>MGASKLRAVLEKLKLSRDDISTAAGMVKGVVDHLLLRLKCDSAFRGVGLLNTGSYYEHVKISAPNEFDVMFKLEVPRIQLEEYSNTRAYYFVKFKRNPKENPLSQFLEGEILSASKMLSKFRKIIKEEINDIKDTDVIMKRKRGGSPAVTLLISEKISVDITLALESKSSWPASTQEGLRIQNWLSAKVRKQLRLKPFYLVPKHAKEGNGFQEETWRLSFSHIEKEILNNHGKSKTCCENKEEKCCRKDCLKLMKYLLEQLKERFKDKKHLDKFSSYHVKTAFFHVCTQNPQDSQWDRKDLGLCFDNCVTYFLQCLRTEKLENYFIPEFNLFSSNLIDKRSKEFLTKQIEYERNNEFPVFDEF[2x]

Cyclic GMP‐AMP synthase (cGAS)* is a sensor of cytosolic double‐stranded DNA (ds‐DNA). ds‐DNA in the cytosol may occur from infection or mitochondrial damage. cGAS is activated by ds‐DNA binding to catalyze the cyclization of ATP and GTP to form a cyclic dinucleotide with mixed 2′,5′‐ and 3′,5′‐phosphodiester linkage (2′,3′‐cGAMP), which in turn activates stimulator of type 1 interferon genes (STING). Activated STING causes the activation of TBK1, which phosphorylates IRF3 allowing it to translocate to the nucleus where it triggers interferon‐inducible gene activation and interferon production. We report here the structure of cGAS with dinucleotides and small molecule inhibitors, and kinetic studies of the cGAS mechanism.

To study the β‐pseudo‐active form we obtained structures of an N‐terminal truncation of cGAS starting at residue 161 (cGAS161)22 in complex with five cyclic dinucleotides (2′,2′‐cGAMP, 2′,3′‐cGAMP, 3′,3′‐cGAMP, 3′,3′‐cdIMP and 3′,3′‐cdUMP), and the linear 2′,5′‐GpAp dinucleotide. In four of these structures, cGAS assumes the β‐pseudo‐active conformation. There is always an interaction between the catalytic acid Asp227 and the dinucleotide when the β‐pseudo‐active conformation occurs. In most cases Asp227 forms a hydrogen bond with the amino group of the guanine base with an approach between 2.5 and 3.3 Å. The exception to this is 3′,3′‐cdIMP which does not have an amino group on its base, but does interact with Asp227 through the 2′‐OH guanine ribose (3.2 Å). Additionally, we observe that in all our cyclic dinucleotides structures, this site had better defined electron density than the other nucleobase site, even for identical ring systems like 3′,3′‐cdIMP and 3′,3′‐cdUMP. Most of these dinucleotides have affinities weaker than 500 μM (the top concentration tested).>MSNYPLHQACMENEFFKVQELLHSKPSLLLQKDQDGRIPLHWSVSFQAHEITSFLLSKMENVNLDDYPDDSGWTPFHIACSVGNLEVVKSLYDRPLKPDLNKITNQGVTCLHLAVGKKWFEVSQFLIENGASVRIKDKFNQIPLHRAASVGSLKLIELLCGLGKSAVNWQDKQGWTPLFHALAEGHGDAAVLLVEKYGAEYDLVDNKGAKAEDVALNEQVKKFFLNNV[2x];>[2x]MERRLIFGTIASKMSLAPEADLDSLIIRND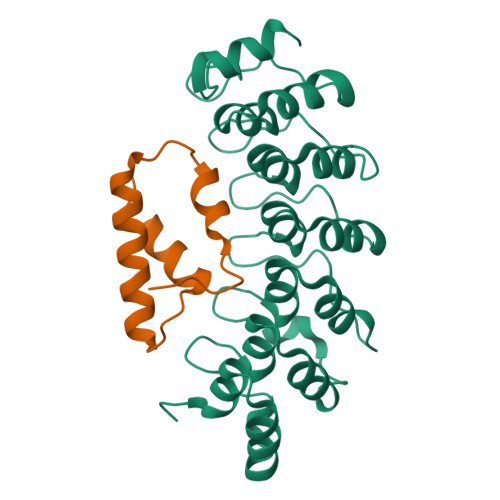SLSGAVIAAIMQEAGLRAVRKNRYVILQSDLEEAYATQVKTDNTVDKFDFYK> ASTTGG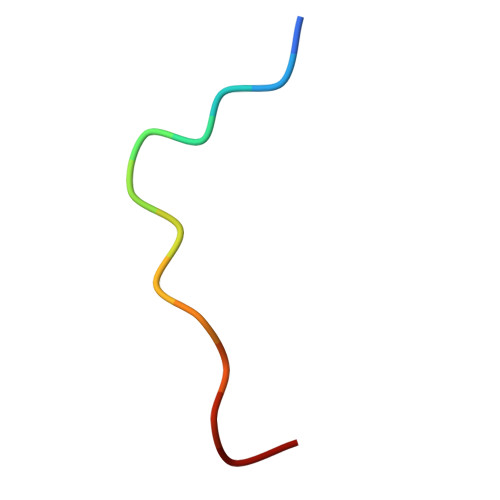NSQRGGG>QTSEYYQEAANPIATNPALWAKVTAPQISWGSTDIRYKKEEPAPIHSAQKSMNLTAWKGEKISAQLVVWTPKVLNDLTFMVSDLTSGSATISKENIRTGFVRYVITDELNKDGLGACGYRNSADFDSTLVADVIDHITPTLTLPANSTQGGWISVNIPQGTKAGKYTGTVTVKADGITLSELKLNLQVKNRTLPPPSEWAFHLDLWQNPYAVSRYYNVEPFSKKHFDLMRPLMKLYADAGGKVITASIMHKPWNGQTYDAFESMVTWLKKADGTWYFDYTVFDKWVEFMMDLGVKKQISCYSMVPWRLSFQYFDQASNSFKFLDAKPGEVAYEEFWMNMLQDFSKHLKAKGWFDITHIAMDERPMKDMQETLKVIRKADKDFKVSLAGTYHKEL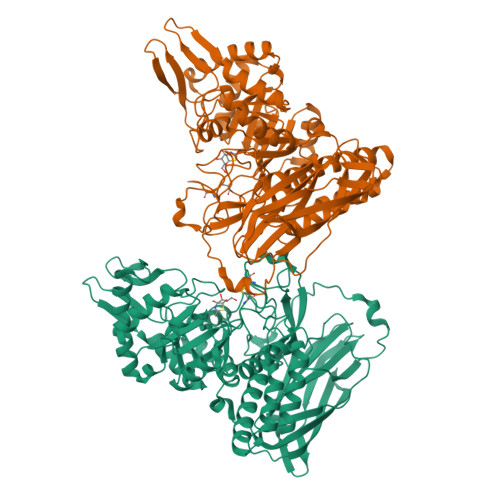LDDLNDYCITIAEKFTPEEIEARRKAGKVTTYYTCCTEPRPNTFTFSEPAEAEWLAWHSAKENLDGYLRWALNSWVKNPLQDSRFTAWAAGDTYMIYPGARSSIRLERLTEGIQFFEKVRILKEEFEEKGNKGAIKNIDKTLKMFDESSMDKISPTTAVNKAKKVINRY[2x]>AECSVDIQGNDQMQFNTNAITVDKSCKQFTVNLSHPGNLPKNVMGHSWVLSTAADMQG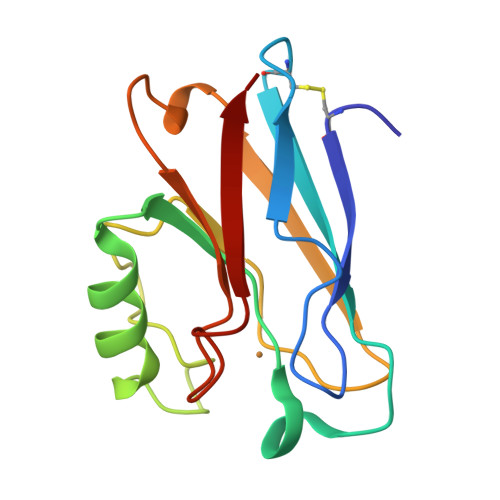VVTDGMASGLDKDYLKPDDSRVIAHTKLIGSGEKDSVTFDVSKLKEGEQYMFFCTNPGHSALMKGTLTLK[4x]>[6x]SESQTLDKVYQMKSKPRGYCLIINNHNFAKAREKVPKLHSIRDRNGTHLDAGAL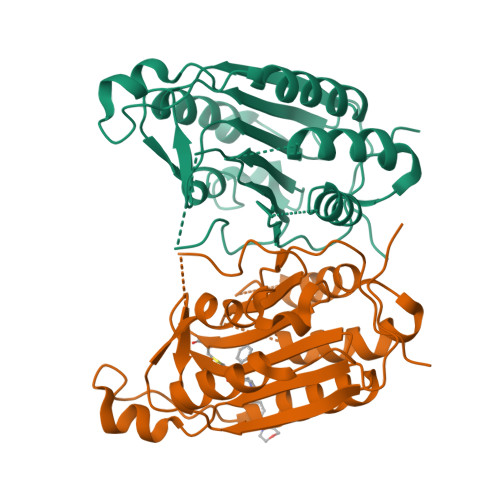TTTFEELHFEIKPHDDCTVEQIYEILKIYQLMDHSNMDCFICCILSHGDKGIIYGTDGQEAPIYELTSQFTGLKCPSLAGKPKVFFIQACQGDNYQKGIPVETASEEQPYLEMALSSPQTRYIPDEADFLLGMATVNNSVSYRNPAEGTWYIQSLCQSLRERSPRGDDILTILTEVNYEVSNKDDKKNMGKQMPQPTFTLRKKLVFPSDAAALEHHHHHH>[4x]GC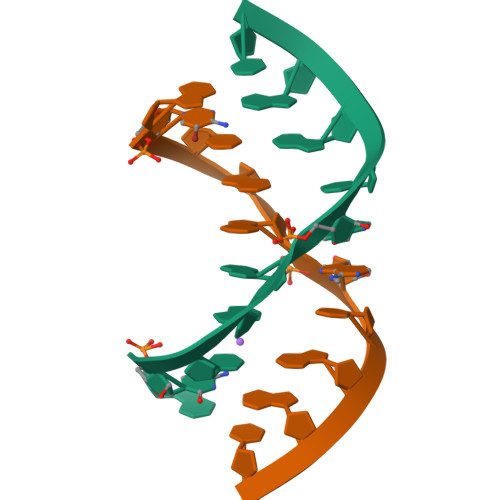CGGAUGGC> AQSVPYGVSQIKAPALHSQGYTGSNVKVAVIDSGIDSSHPDLKVAGGASMVPSETNPFQDNNSHGTHVAGTVAALNNSIGVLGVAPSASLYAVKVLGADGSGQYSWIINGIEWAIANNMDVINMSLGGPSGSAALKAAVDKAVASGVVVVAAAGNEGTSGSSSTVGYPGKYPSVIAVGAVDSSNQRASFSSVGPELDVMAPGVSIQSTLPGNKYGAYNGTSMASPHVAGAAALILSKHPNWTNTQVRSSLENTTTKLGDSFYYGKG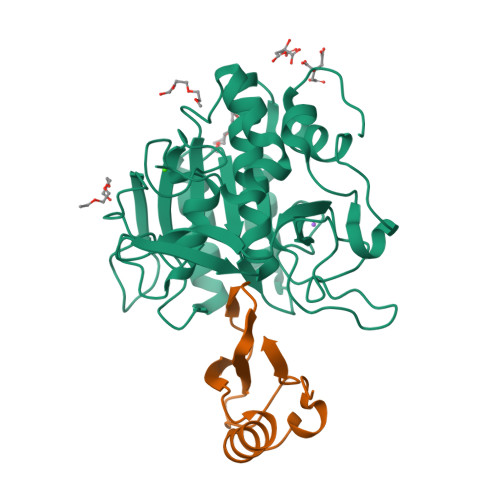LINVQAAAQHHHHHH;> MKTEWPELVGKSVEEAKKVILQDKPAAQIIVLPVGTIVTGEYRIDRVRLFVDRLDNIAQVPRVG3'-DEOXY 3'-AMINO ADENOSINE-5'-DIPHOSPHATE 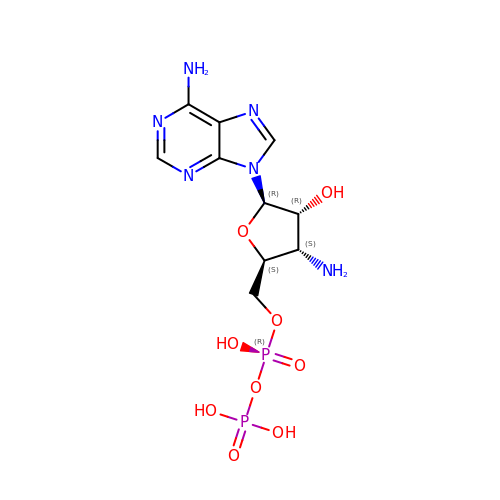| C10 H16 N6 O9 P2 | VKODIDNZKBYXJO-QYYRPYCUSA-N> GSTTPLLANSLSVHQLAAQGEMLYLATRIEQENVINHTDEEGFTPLMWAAAHGQIAVVEFLLQNGADPQLLGKGRESALSLACSKGYTDIVKMLLDCG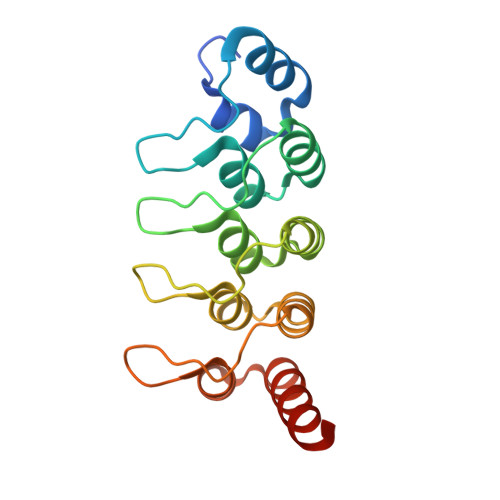VDVNEYDWNGGTPLLYAVHGNHVKCVKMLLESGADPTIETDSGYNSMDLAVALGYRSVQQVIESHLLKLLQNIKE> GSHMKILVINGPNLNFLGIREKNIYGNENYEYLVNMINEYCKSKNIEVECYQSNHEGAIIDKIQEAYFNGTDGIVINPGAYTHYSYAIRDA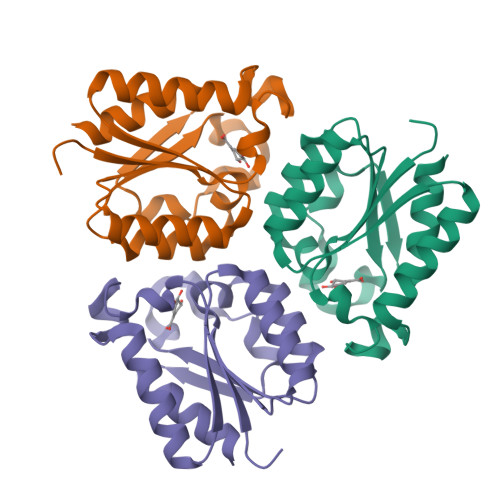LASVSHIKKIEVHISNVNEREEFRHISVTEPVCNGQIVGQGLKGYIMAIDMLNS>MADKKTDIPTLIADSTKASLQDFNHDYGKQWTFGENWSNVNTMFETYVNKYLFPKINETLLIDIALGNRFNWLAKEQDFIGQYSEEYVIMDTIPIEMNLSKSEELMLKRNYPQMATRLYGSGIVKKQKFTLNNNDVRFNFQTLGDATNYALGVLRKKISDINVQEEKEIRAMMVDYAINQLQDSNRRTASSKEDLTERVFEAILNMQNNSAKYNEVHKASGGSVGQYTTVSKLSDIAILTTDSLKSYLLDTKIANTFQMAGIDFTDHIISFDDLGGVYKTTKDVTLANEDTINYLRAFGDYQAMIGDVIPTGSVFTFNVSDLKEFKGNIEEIKPQGELFAFIFDINALKYKRNTKGMLKEPFYNGEFDEVTHWIHYYSFKAMSPFFNKILITEAPKEQPDAGATE[4x];>MANFDGNEMRGMTHANYEDSRLNKSRELNANMSIGTSKSEDEYGRQVHSLTKQSYSDDSVQEA[4x]

Staphylococcal picoviruses are a group of strictly lytic, short-tailed bacteriophages with compact genomes that are attractive candidates for therapeutic use. Here, we report the structure of the complete virion of S. epidermidis–infecting phage Andhra, determined using high-resolution cryo–electron microscopy, allowing atomic modeling of 11 capsid and tail proteins. The overall structure of the Andhra virion follows that of other phages in this group, with an isometric head (capsid) around 500 Å in diameter (vertex to vertex), connected to a 400-Å-long, straight tail surrounded by 12 appendages. The head has icosahedral symmetry, with the tail attached to a portal structure located at 1 of the 12 fivefold vertices.

The capsid is a T = 4 icosahedron containing a unique stabilizing capsid lining protein. The capsid has T = 4 architecture and is composed of 240 copies of the major capsid protein (CP), gene product (gp) of ORF18 (gp18), arranged into 12 pentamers located on the fivefold axes and 20 hexamers located on the twofold axes. In addition, there are 240 copies of a small 63-residue protein, gp19, that we refer to as the “capsid lining protein” (CLP). There are thus four copies of CP in the icosahedral asymmetric unit, labeled A to D, with A forming the pentamers and B to D forming the hexamers, and four copies of CLP, labeled E to H. The Andhra CP (405 residues) has the expected HK97-like fold found in all Caudovirales, consisting of an N-arm (residues 1 to 82), an E-loop (83 to 122), a P-domain (123 to 180 and 344 to 386) featuring a long “spine” α helix, and an A-domain (181 to 343 and 387 to 395). There is a 62-residue insertion (I-domain) into the A-domain (residues 276 to 328) that forms 240 prominent protrusions on the surface of the shell. CLP (gp19) forms an S-shaped loop that lines the inside of the capsid. For subunits F to H, the N-terminal 28 residues form a hook-like structure that interacts with the A-domain of a CP subunit. The chain then passes underneath the neighboring subunit within the hexamer and forms a small α helix that connects to a CP subunit in the adjacent capsomer. For subunit E, which starts in the pentamer (CP subunit A), only residues 31 to 53, which connect with a D subunit in the hexamer, were seen.>MENLKKYLEVAKIAALAGGQVLKENFGKVKKENIEEKGEKDFVSYVDKTSEERIKEVILKFFPDHEVVGEEMGAEGSGSEYRWFIDPLDGTKNYINGFPIFAVSVGLVKGEEPIVGAVYLPYFDKLYWGAKGLGAYVNGKRIKVKDNESLKHAGVVYGFPSRSRRDISIYLNIFKDVFYEVGSMRRPGAAAVDLCMVAEGIFDGMMEFEMKPWDITAGLVILKEAGGVYTLVGEPFGVSDIIAGNKALHDFILQVAKKYMEVAV[4x]

The riboflavin biosynthetic pathway is well-studied with dedicated enzymes to perform complex chemical transformations, with the exception of an unknown phosphatase that catalyzes the dephosphorylation of ARAPDP, the product of RibD, to generate 5-amino-6-ribitylamino-pyrimidinedione (ARAPD), the substrate for lumazine synthase. Using an anaerobic activity-based screen, two phosphatases from Aquifex aeolicus were identified that dephosphorylate ARAPDP, but only one reconstitutes riboflavin production in a one-pot experiment with the other four enzymes of riboflavin biosynthesis. The structures of both enzymes were determined by X-ray crystallography to reveal the vastly different folds capable of performing the ARAPDP dephosphorylation chemistry.

The first enzyme, annotated as an IMP, is nonspecific, and indiscriminately dephosphorylates ARAPDP along with ribulose 5-phosphate and NADPH, two required substrates of riboflavin biosynthesis. IMP is reported as an IMP, which is a member of the phosphodiesterase family of enzymes and shares significant homology to the putative target for lithium therapy as a mood stabilizer. The structure determined here was solved to 1.75 Å with two homodimers in the asymmetric unit. Inositol monophosphatases are reported to fold as a α/β/α/β/α penta-layered sandwich that assemble as homodimers. IMP displays that standard fold and PDBePISA calculates an interface surface area of greater than 1700 Å2 between the A and B chains, consistent with stable dimer formation. In addition, the estimated molecular weight in solution was that of a dimer as determined by preparative gel filtration chromatography during purification. Density was observed in the active site for metal ions, but no metals were added during purification or crystallization; therefore, these ions were derived from the heterologous enzyme production in E. coli. Inductively coupled plasma mass spectrometry (ICPMS) was used to unambiguously determine that magnesium is bound to the protein. Whereas reported myo-inositol phosphatase structures have three metals modeled in the active site, the electron density in the IMP active site only supported modeling of two magnesium ions. IMP is unable to facilitate riboflavin formation in combination with the rest of the pathway's enzymes from initial substrates GTP, NADPH, and Ru5P as it indiscriminately dephosphorylates NADPH and Ru5P.> NEFD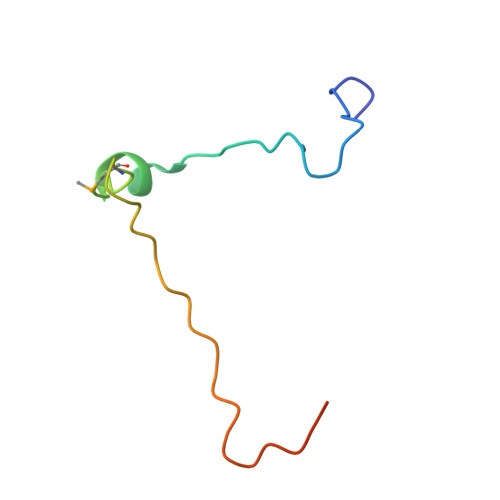RIIENQEKSLKASKSTPDGTIKDRRLFMHHVSLEPITTVPFRTTKERQENLYFQG Pygo contains a single zinc-coordinated PHD finger in its C-terminus, by which it binds directly to a short Lgs domain [called homology domain 1 (HD1)]; Lgs in turn uses its homology domain 2 to bind to Armadillo, thus forming a ‘chain-of-adaptors’.7,10 How Pygo and Lgs assist Armadillo as a transcriptional co-activator is unclear. Vertebrates have two orthologs of Pygo and Lgs: Pygo1 and Pygo2, and BCL9 and BCL9-2/B9L (referred to as B9L), which contribute to efficient β-catenin-dependent transcription in human colorectal cancer cell lines with high Wnt pathway activity. To our knowledge, Pygo PHD fingers are the only ones whose histone H3 tail binding is regulated by a co-factor ligand, namely, the HD1 of BCL9 proteins: human BCL9 HD1 significantly increases the affinity of human Pygo1 PHD for H3K4me, while Lgs HD1 is essential for H3K4me binding of Drosophila Pygo PHD. Here, we explore the molecular mechanism by which mammalian HD1 assists PHD in binding to histone H3 tail.

Given the emerging physiological differences between the murine Pygo paralogs and the murine Bcl9 paralog, we measured the binding affinities of all four PHD and HD1 combinations for dimethylated histone H3 tail peptide (H3K4me2) by isothermal titration calorimetry (ITC) and found that the complex between Pygo2 PHD and B9L HD1 (PHDPygo2–HD1B9L) has the highest affinity for H3K4me2. To further explore the underlying molecular mechanism of this communication, we solved the crystal structure of the human PHDPygo2–HD1B9L complex. The purified complex yielded crystals under multiple conditions, and its structure was solved at 1.9 Å resolution. The overall structure is very similar to that of PHDPygo1–HD1BCL9 (with a 0.593 Å rmsd for the core Cα backbone  compared to that of 2VPB13). Like other PHD fingers, PHDhPygo2 binds to two Zn2+ in a cross-braced conformation involving two pairs of anti-parallel β-strands, followed by an α-turn and another β-strand flanked by two α-helices. It exhibits two distinct protein-interacting surfaces on opposite sides: one for histone binding and another for HD1 binding. HD1B9L is a compact domain that consists of an N-terminal β-strand, followed by two α-helices connected by a short loop that allows folding back of α2 towards α1. The main difference between the structure shown here and that of the PHDPygo1–HD1BCL9 complex is the presence of an extra helix (α2) in B9L HD1 that was not properly formed in previous structures, perhaps as a result of crystal contacts. Secondly, α2 is positioned so that I258 and L259 are in contact with the base of the A1 pocket, namely, with PHD residues T371-A375, which flank the connecting loop between α1 and β5, apparently buttressing the pocket. α2 is thus an essential structural feature of HD1B9L, directly supporting the A1 pocket base of PHDPygo2.

>GLVYPCGACRSEVNDDQDAILCEASCQKWFHRECTGMTESAYGLLTTEASAVWACDLCLKTKEGSGSGSGSQFVYVFTTHLANTAAEAVLQGRADSILAYHQQNV[2x]> NLSLSQSNF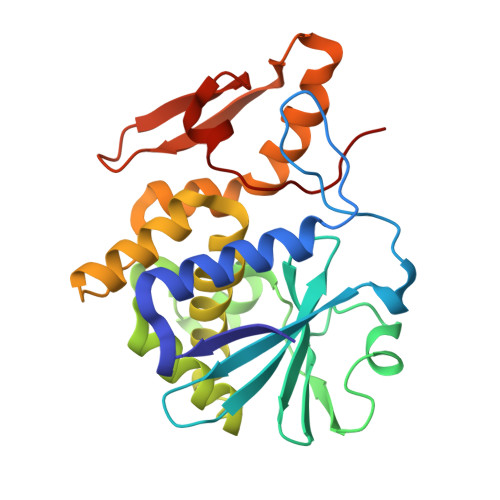SADTYKSFIKNLRKQLTIGASYGSAGIPILKHSVPICERFLLVDLTNGDNETITLAINVEDAGFAAYRAADRSYFFQNAPPIASYVIFTDTNQNIMNFNNTFESIEIVGGTTRSETPLGIMHFEASIFHLFVHDENYVPTSFLVLIQMVLEAAKFKFIEQKVIHSIMDMEDFTPGLAMLSLEENWTQLSLQLQASESLNGVFGDSVSLYNSMDEPIGVDSMYYPILTANMAFQLYQCP> MLSKRLLNFESFEVMDILALAQKLESEGKKVIHLEIGEPDFNTPKPIVDEGIKSLKEGKTHYTDSRGILELREKISELYKDKYKADIIPDNIIITGGSSLGLFFALSSIIDDGDEVLIQNPCYPCYKNFIRFLGAKPVFCDFTVESLEEALSDKTKAIIINSPSNPLGEVIDREIYEFAYENIPYIISDEIYNGLVYEGKCYSAIEFDENLEKTILINGFSKLYAMTGWRIGYVISNDEIIEAILKLQQNLFISAPTISQYAALKAFEKETEREINSMIKEFDRRRRLVLKYVKDFGWEVNNPIGAYY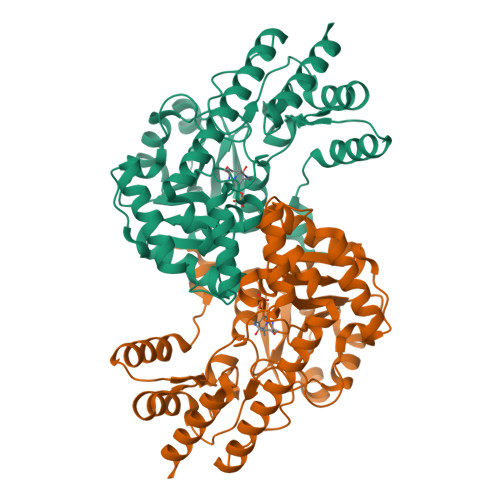VFPNIGEDGREFAYKLLKEKFVALTPGIGFGSKGKNYIRISYANSYENIKEGLERIKEFLNK> GSAMGSSTSTSRATYMDRFNIPKNHVDLIWDKDGTKSHTRGNTTYRWTERKSNVGVYVGYSEMYDSSAQAYCQSSSAKIDTKTTVGAPYMAAGACPNYGKVIAFTKRDGSRSDMTRWKNEIHANVMPHSTTSCASRADPGAAEVAKSIEGFAMYAGYLTHCPYNVNVYRQDMVTDKEFDSTVCNFVTESNPLRFLDTTQRQSTQPYTEYAFHGKGGHKGYDYKGQTSHVGCPPYNPPHVTKGMKDSSWITGPFECSILSRCTTHCWPYKSGGNCFRSLPAMFDMSTGECRLLGYHTQDFR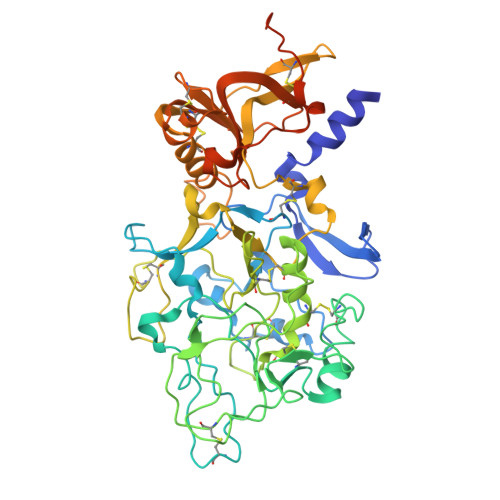SSTCAELTTDDTNAFYCVRPMKTAASSNMVYVTSHTRPDHETKCPPREPLKNVRWGVVSKGKYCKPMNARASLSNATAEQCGQRLFMLSSADGSSLSSQVRGYHWATFVATDCNMGESCAATARGKCFFYSTVPECLIHSPTTMAFTSLSAVDPSIAIDPDSIAVLPEDKCVSVDCGAHGTCDVATGKCVCEPGFTGERCDAAALVPR> GSMAEGSAVSDPQHAARLLRALSSFREESRFCDAHLVLDGEEIPVQKNILAAASPYIRTKLNYNPPKDDGSTYKIELEGISVMVMREILDYIFSGQIRLNEDTIQDVVQAADLLLLTDLKTLCCEFLEGCIAAENCIGIRDFALHYCLHHVHYLATEYLETHFRDVSSTEEFLELSPQKLKEVISLEKLNVGNERYVFEAVIRWIAHDTEIRKVHMKDVMSALWVSGLDSSYLREQMLNEP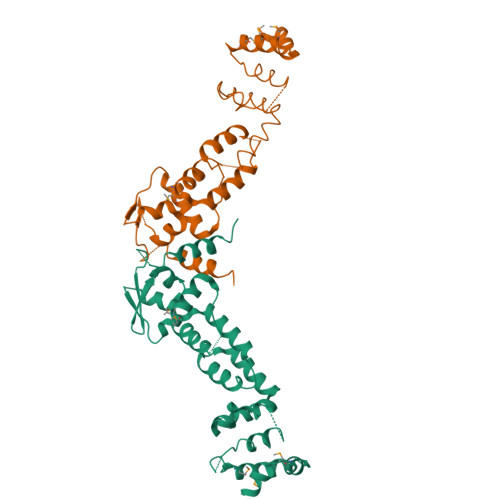LVREIVKECSNIPLS;> GSMAEGSAVSDPQHAARLLRALSSFREESRFCDAHLVLDGEEIPVQKNILAAASPYIRTKLNYNPPKDDGSTYKIELEGISVMVMREILDYIFSGQIRLNEDTIQDVVQAADLLLLTDLKTLCCEFLEGCIAAENCIGIRDFALHYCLHHVHYLATEYLETHFRDVXXXXXXXXXXXXXXXXXXXXXXXXXXXXXXXXXXXXXXXXXXXXXXKVHMKDVMSALWVSGLDSSYLREQMLNEPLVREIVKECSNIPLS> GSFTSHQVAGHMYGKDKVGILQHPDGTVLKQLQPPPRGPRELEFYNMVYAADCFDGVLLELRKYLPKYYGIWSPPTAPNDLYLKLEDVTHKFNKPCIMDVKIGQKSYDPFASSEKIQQQVSKYPLMEEIGFLVLGMRVYHVHSDSYETENQHYGRSLTKETIKDGVSRFFHNGYCLRKDAVAASIQKIEKILQWFENQKQLNFYASSLLFVYEGSSQGGSGGEVEVRMIDFAHVFPSNTIDEGYVYGLKHLISVLRSILDN

Inositol polyphosphate multikinase (IPMK) is a ubiquitously expressed kinase that has been linked to several cancers, − and loss of IPMK kinase activity in cells decreases cell growth and proliferation in several human cell lines. The first crystal structure of any IPMK orthologue published was that of the yeast ipk2, followed by the plant Arabidopsis thaliana orthologue. These structures established that IPMK has the typical kinase fold, containing an N-terminal lobe and a C-terminal lobe with the ATP-binding site at the interface between these two lobes. Here, we solved the X-ray crystal structures of 14 of this new generation of compounds complexed with the kinase domain of human IPMK. The structures solved here show a polar contact cluster in this region, which together with essential polar contacts from the hinge region suggests the two-point anchoring ligand binding mechanism proposed here to synergistically enhance the potency of the IPMK inhibitors.

Compound 1 IC50 values suggest more potency toward IPMK (IC50 = 12.8 nM) than either of the related kinases IP3K-A (IC50 = 8000 nM) or IP6K1 (IC50 = 146 nM), with compound 1 having approximately 10-fold selectivity for IPMK over IP6K1. Compound 1 directly bound IPMK with K d = 11 nM by isothermal titration calorimetry, consistent with the IC50 value. Compound 1 contains three chemical moieties: the benzisoxazole ring that we call the core, with moieties A (acrylic acid) and B (dimethylphenyl) on either side. The core of compound 1 formed four hydrogen bonds with the IPMK hinge region, including three hydrogen bonds with IPMK backbone residues and one hydrogen bond with the carboxylic group of Asp132. The crystal structure of compound 1 with IPMK also revealed that moiety A penetrated a subpocket that is contoured by three hydrophobic IPMK residues (Leu130, Iso384, and Phe386). The four polar amino acids in the IPMK back pocket (Lys75, Glu86, Tyr90, and Asp385) also formed a hydrogen bond network with moiety A of compound 1. Thus, we named residues Lys75, Glu86, and Tyr90 the “KEY motif,” with this motif specific to inositol phosphate kinases. Together with the hinge region, IPMK anchored compound 1 with two hydrogen bond clusters, suggesting a two-point anchoring recognition mechanism. The core of compound 1 also forms several hydrophobic interactions with residues Ile65, Val73, Pro111, and Leu254 of IPMK, also observed in the complex of ATP with IPMK. In addition, Leu130, Ile384, and Phe386 are close enough to form van der Waals contacts with moiety A. For moiety B, Gln67, Thr134, Ile142, Asp144, and Leu254 are within van der Waals contact range.>[2x]MRGSHHHHHHGSRVYENKEELKSEINKTFEKYIAEFDNIPESLKDKRIDEVDRTPAENLAYQVGWTTLVLKWEEDERNGLQVKTPSDEFKWNQLGELYQWFTDTYAYLSLQELKSKLNENINSIYVMIDSLSDEELFKPHMRKWADDATKTAVWEVYKFIHVNTVAPFKTFRNKIRKWKKIVL

The precursor PdDfsB is cleaved by subtilisin to yield biologically active Slf, and the chemical gradients of both proteins between two growing colonies could be accurately modelled. However, remarkably, the dfsB gene is widely distributed across Gram-positive and to some extent Gram-negative bacterial kingdoms (PFAM entry DUF1706). PdDfsB adopts a four-helical bundle core structure that belongs to the DinB structural superfamily. The most strongly conserved region of PdDfsB is the C-terminal helix, which is present within the mature Slf sequence.

We were able to express, purify and obtain crystal structures for DfsB homologues from Clostridium difficile 630 and Escherichia coli UTI89, as well as of IRC4 from S. cerevisiae. For the purposes of clarity, we refer to the first two proteins as CdDfsB and EcDfsB, respectively; however, we have no evidence that they are truly acting as DfsB homologues by undergoing cleavage and release of their analogous Slf “toxin”. The overall structures of CdDfsB, EcDfsB and IRC4 are identical with that of PdDfsB, with strong conservation of overall topology and surface charge, particularly in the C-terminal helix. We solved the crystal structure of a S. agalactiae DfsB dimer (SaDfsB) by molecular replacement using a pruned CdDfsB structure as the search model.2,6-bis(methylamino)-1,7-dihydro-8H-imidazo[4,5-g]quinazolin-8-one | C11 H12 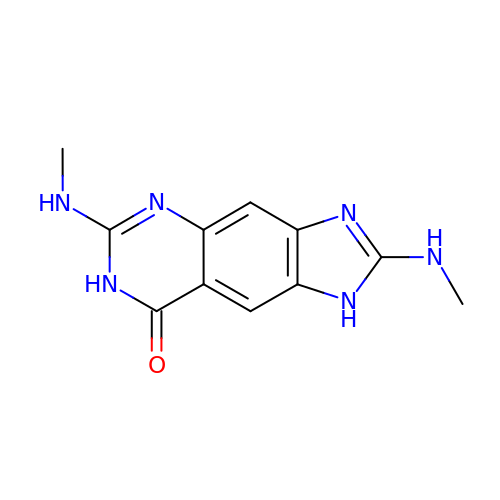N6 O | YOTQNVNIJNKFAK-UHFFFAOYSA-N>[2x]MKESRAKKFQRQHMDSDSSP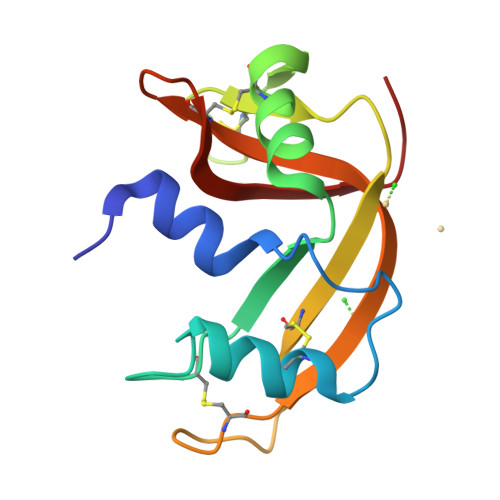SSSSLYCNLMMLLRNMTQGRCKPVNTFVHEPLVDVQNVCFQEKVTCKNGQGNCYKSNSSMHITDCRLTNGSRYPNCAYRTSPKERHIIVACEGSPYVPVHFDASVEDST> MGHHHHHHHHHHSSGHIEGRHMDINGVLLLDKPQGMSSNDALQKVKRIYNANRAGHTGALDPLATGMLPICLGEATKFSQYLLDSDKRYRVIARLGQRTDTSDADGQIVEERPVTFSAEQLAAALDTFRGDIEQIPSMYSALKYQGKKLYEYARQGIEVPREARPITVYELL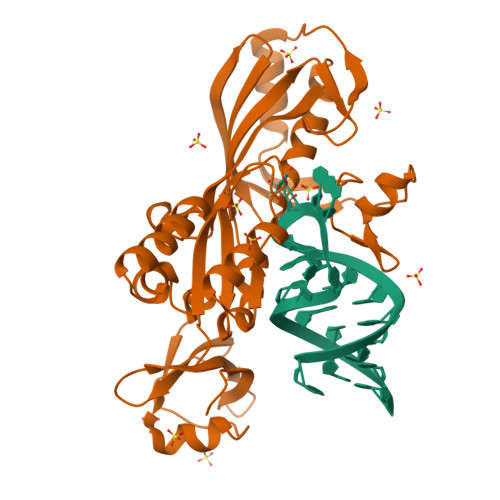FIRHEGNELELEIHCSKGTYIRTIIDDLGEKLGCGAHVIYLRRLAVSKYPVERMVTLEHLRELVEQAEQQDIPAAELLDPLLMPMDSPASDYPVVNLPLTSSVYFKNGNPVRTSGAPLEGLVRVTEGENGKFIGMGEIDDEGRVAPRRLVVEYPA>[4x]MNDTAGELEFVPLAANDDETVGQWLDLMALAAETGPRAAPPCNVDMVGSLRFAPPATALDDWVVRSGGR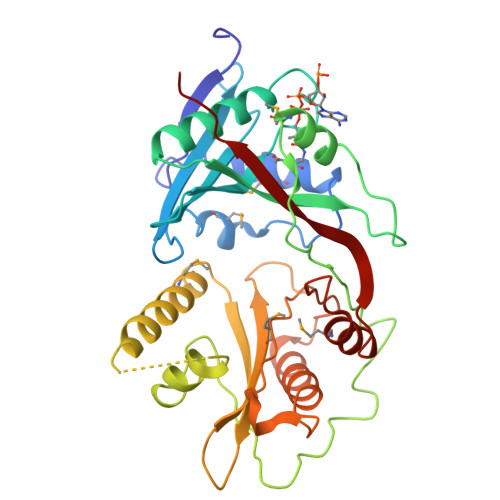VVGALRLALPDGAPTARVDQLLVHPGRRRRGIGRALWAHARELARKHDRTTLTATVVESLPSGPAQDPGPAAFAAAMGAHRSDIPAGTHQWLDLDRHDPLADGVPAVPAGYSLVTWGTITPDEYAVPVSELELSLGAGPVDRAAQEVRTSYARQFETMRVGRGRRAYHTGAVHDATGALAGYTSVSKTTGNPAYALQGMTVVHREHRGHALGTLLKLANLEYVLRHEPEVRLVETANAEDNHPMIAVNAALGFEPYDRWVFWTAEAGPSD>GVLPVEKCNLEDSACMTSAFQQALPTFVAGLPDHGVEVMDVLDLDDFAFDLSGLQFTLKEGKLKGLKGAVIDNVKWDLKKKNIEVDFHLDATVKGHYTAGGRILILPITGDGQMKLKLKNIHIHLVVSYEMEKDAEGVDHVIFKKYTVTFDVKDNAQFGLTNLFNGNKE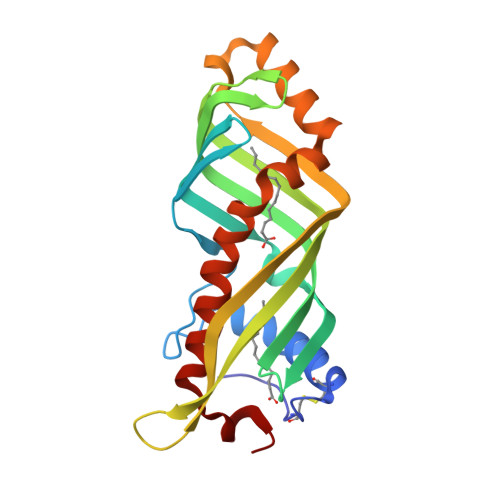LSDTMLTFLNQNWKQVSEEFGKPVMEAAAKKIFKNIKHFLAKVPIAEIANV[2x]>[2x]MASRGLDLWLDEHVWKRKQEIGVKGENLLLPDLWLDFLQLSPIFQRKLAAVIACVRRLRTQATVYPEEDMCMAWARFCDPSDIKVVILGQDPYHGGQANGLAFSVAYGFPVPPSLRNIYAELHRSLPEFSPPDHGCLDAWASQGVLLLNTILTVQKGKPGSHADIGWAWFTDHVISLLSERLKACVFMLWGAKAGDKASL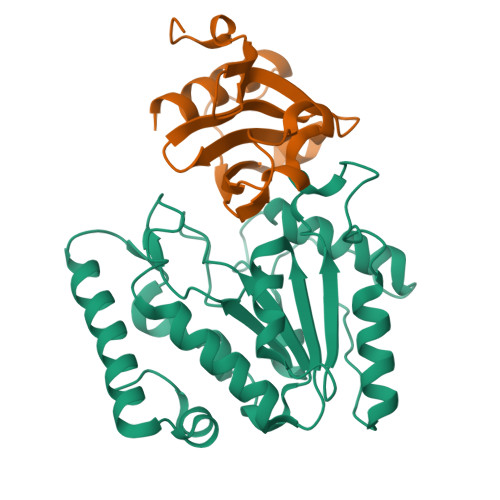INSKKHLVLTSQHPSPLAQNSTRKSAQQKFLGNNHFVLANNFLREKGLGEIDWRL;>MTLELQLKHYITNLFNLPKDEKWECESIEEIADDILPDQYVRLGALSNKILQTYTYYSDTLHESNIYPFILYYQKQLIAIGYIDENHDMDFLYLHNTIMPLLDQRYLLTGGQ[2x]>[4x]GSMTGASTTTATMRQRWQAVMMNNYGTPPIALASGDGAVVTDVDGRTYIDLLGGIAVNVLGHRHPAVIEAVTRQMSTLGHTSNLYATEPGIALAEELVALLGADQRTRVFFCNSGAEANEAAFKLSRLTGRTKLVAAHDAFHGRTMGSLALTGQPAKQTPFAPLPGDVTHVGYGDVDALAAAVDDHTAAVFLEPIMGESGVVVPPAGYLAAARDITARRGALLVLDEVQTGMGRTGAFFAHQHDGITPDVVTLAKGLGGGLPIGACLAVGPAAELLTPGLHGSTFGGNPVCAAAALAVLRVLASDGLVRRAEVLGKSLRHGIEALGHPLIDHVRGRGLLLGIALTAPHAKDAEATARDAGYLVNAAAPDVIRLAPPLIIAEAQLDGFVAALPAILDRAVGAP

The L-arginine biosynthesis pathway consists of eight enzymes that catalyse the conversion of L-glutamate to L-arginine, appears to be attractive target for anti-Tuberculosis (TB) drug discovery. The arginine biosynthesis pathway consists of eight different enzymes ([Fig fig1]) all considered to be essential for *M. tuberculosis* growth *in vitro*. In this work, the ligandability of four enzymes of the pathway ArgB, ArgC, ArgD and ArgF is explored using a fragment-based approach. In conclusion, using a fragment-based approach, we have discovered inhibitors that bind to novel sites in ArgB and ArgF and to the active sites of ArgC and ArgD, which in case of ArgB show on target activity against *M. tuberculosis*.

The first crystal structure of the ArgD holoenzyme from *M. tuberculosis* obtained ([Fig fig3]) showed that the protomer has three domains: the smaller N-terminal segment (residues 7 to 74), the relatively larger C-terminal domain (residues 286 to 396), and the central PLP-binding domain (residues 85 to 273), which is also the largest and has a Rossmann-like overall fold ([Fig fig3]). The prosthetic group PLP is covalently linked to Lys253 via an aldimine linkage. While NMR608 was the only hit validated by all techniques the fragment library contained a compound with similar structure (NMR868) that had only a melting shift of 0.9 C and therefore wasn’t selected initially for further testing. However, soaking of this fragment revealed that it binds in almost the same position as NMR608 ([Fig fig3]). Nevertheless, The orientation of the acid group is slightly different in NMR868 and it no longer interacts directly with arg142. For ArgD selectivity might be more difficult to achieve since many of the active site residues are conserved in comparison with the human cytoplasmic and mitochondrial enzymes.Cyclic GMP-AMP (cGAMP) synthase (cGAS) is essential for the host defense against cytosolic double-stranded (ds)DNA arising from various maladies (e.g., pathogen invasion, ionizing irradiation, and genotoxic chemicals). Upon directly binding to and dimerizing on dsDNA, cGAS cyclizes ATP and GTP into 2′−5′/3′−5′-linked cGAMP, a unique metazoan second messenger for initiating type-I interferon (IFN-I)-mediated inflammatory responses. cGAS is central to antitumor immunity, host defense against an array of pathogens, and regulating autoimmunity. Here, we resolve these numerous fundamental mechanistic questions in innate immunology and present a unifying catalytic mechanism of cGAS. Finally, we reveal how mouse cGAS achieves more stringent substrate selectivity and higher catalytic efficiency than the human enzyme. Together, we set forth a unifying catalytic mechanism of cGAS in which dsDNA-binding pre-organizes the active site into a rigid yet adaptable lock for two sets of keys (substrates and intermediate) necessary to specifically synthesize 2′−5/3′−5′-cGAMP.

To test whether such a precise NTP-specific coordination is critical for cyclization, we soaked Mg2++ITP/GTP, ATP/ITP, or GTP alone into WT-mcGAScat•dsDNA, all of which produced respective linear dinucleotides bound at the active site. Next, we identified pppIpA based on how the nucleoside at Site-2 resembles the adenine of pppGpA; Arg364 was also pushed away as seen from pppGpA and the 3′-OH was in position for catalysis. Nevertheless, the second Mg2+ was again missing, and the α-phosphate of pppIpA appeared misaligned compared to pppGpA (bottom). These observations suggest that the H-bond between the α-phosphate and the -NH2 of guanine is important for positioning the metal•intermediate complex for cyclization. C–E Comparing pppGpA-bound QN-mcGAScat•dsDNA vs. WT-mcGAScat•dsDNA bound to pppGpI (C), pppIpA (D), and pppGpG (E). Importantly, our results consistently indicate that any deviations from such a precise coordination would prevent cyclization: any misalignments of the 3′-OH nucleophile (pppGpI) or the α-phosphate electrophile (pppIpA) would disrupt catalytic metal binding, and the enzyme-mediated intra-dinucleotide interactions would trap pppGpG in a nonproductive state.

>[2x]GTGPDKLKKVLDKLRLKRKDISEAAETVNKVVERLLRRMQKRESEFKGVEQLNTGSYYEHVKISAPNEFDVMFKLEVPRIELQEYYETGAFYLVKFKRIPRGNPLSHFLEGEVLSATKMLSKFRKIIKEEVKEIKDIDVSVEKEKPGSPAVTLLIRNPEEISVDIILALESKGSWPISTKEGLPIQGWLGTKVRTNLRREPFYLVPKNAKDGNSFQGETWRLSFSHTEKYILNNHGIEKTCCESSGAKCCRKECLKLMKYLLEQLKKEFQELDAFCSYHVKTAIFHMWTQDPQDSQWDPRNLSSCFDKLLAFFLECLRTEKLDHYFIPKFNLFSQELIDRKSKEFLSKKIEYERNNGFPIFDKL S,3-HYDROXYBUTAN-2-ONE | C4 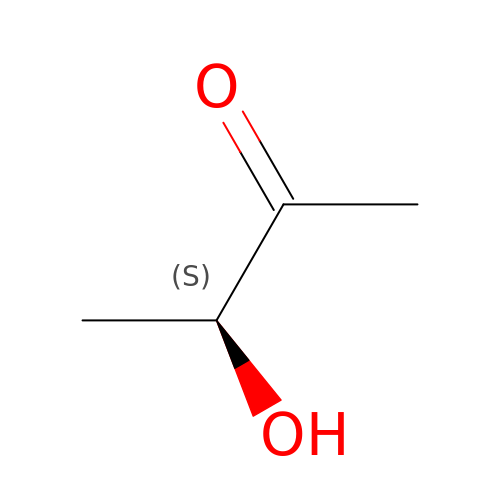H8 O2 | ROWKJAVDOGWPAT-VKHMYHEASA-N>[2x]EQARPADDALAALGAQLFVDPALSR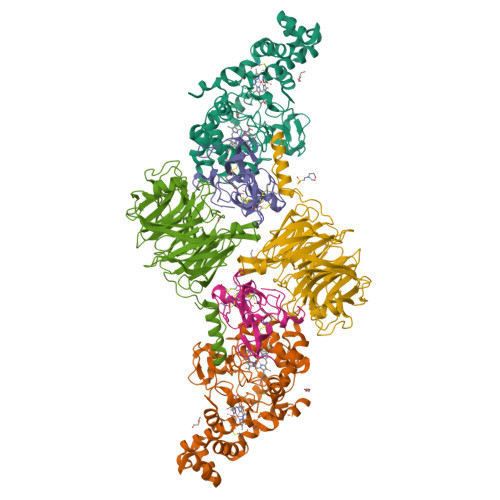NATQSCATCHDPARAFTDPREGKAGLAVSVGDDGQSHGDRNTPTLGYAALVPAFHRDANGKYKGGQFWDGRADDLKQQAGQSMLNPVEMAMPDRAAVAARLRDDPAYRTGFEALFGKGVLDDPERAFDAAAEALAAYQATGEFSPFDSKYDRVMRGEEKFTPLEEFGYTVFITWNCRLCHMQRKQGVAERETFTNFEYHNIGLPVNETAREASGLGADHVDHGLLARPGIEDPAQSGRFKVPSLRNVAVTGPYMHNGVFTDLRTAILFYNKYTSRRPEAKINPETGAPWGEPEVARNLSLAELQSGLMLDDGRVDALVAFLETLTDRRYEPLLEESRAAQKDHHHHHH;>[2x]ADAPAGTDPRAKWVPQDNDIQACDYWRHCSIDGNICDCSGGSLTNCPPGTKLATASWVASCYNPTDGQSYLIAYRDCCGYNVSGRCPCLNTEGELPVYRPEFANDIIWCFGAEDDAMTYHCTISPIVGKASHHHHHH;>QDAPEAETQAQETQGQAAARAAAADLAAGQDDEPRILEAPAPDARRVYVNDPAHFAAVTQQFVIDGEAGRVIGMIDGGFLPNPVVADDGSFIAHASTVFSRIARGERTDYVEVFDPVTLLPTADIELPDAPRFLVGTYPWMTSLTPDGKTLLFYQFSPAPAVGVVDLEGKAFKRMLDVPDCYHIFPTAPDTFFMHCRDGSLAKVAFGTEGTPEITHTEVFHPEDEFLINHPAYSQKAGRLVWPTYTGKIHQIDLSSGDAKFLPAVEALTEAERADGWRPGGWQQVAYHRALDRIYLLVDQRDEWRHKTASRFVVVLDAKTGERLAKFEMGHEIDSINVSQDEKPLLYALSTGDKTLYIHDAESGEELRSVNQLGHGPQVITTADMG[2x]>[2x]ATSMSFVIWITGPSG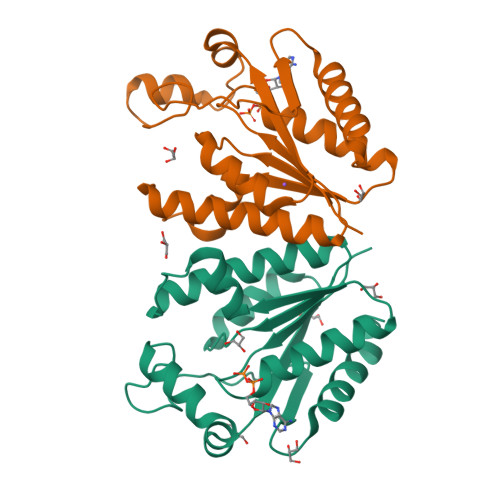AGKTTLANALYKKLESMGYRVELLDGDGVRRKLYPNLGFSEEERWMHNRVVVEMARRLSRNGIITIVSVVSPYRAWREYARKEIEKFVEVYPRCPLEVRMKRDPKGLYSKALRGEIKGLTGLDGEYEEPENPEVVVDTDKMTVEEEVEAVLKKLMELGYL> MFGLASKGFINTSLVMVPQMNFGANLKQLKIRMKAIGSIKKITKAMKMVAASKMKAETSRLENGRNFAVGSVQKMLENESYVQKKKSTTAPKSTLLVPITSDKGLCGSVNSSIVREVKRLALNNRSAFGLLPVGEKGSSGLSR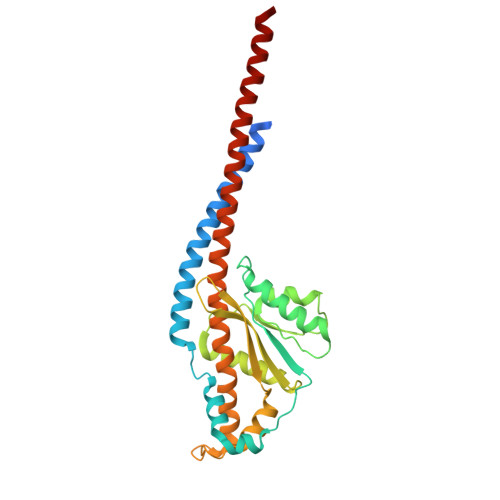PFPDLLKSSIVNIQNVNFPTAAAIAHQVSTQGAGYDQVTLIYNHFKNAISYVVKHQELLPRAQFLNLFKYVTRHEAVEPELEYSKNYFFELYMASSVYNALLNSSASEQASRMNAMENASKNAGEILSKLTLDYNKARQAKITMELIEIISGASIV> MWSHPQFEKGSMELSYATTMHYRDVVFYVTTDRNRAYFVCGGCVYSVGRPCASQPGEIAKFGLVVRGTGPDDRVVANYVRSELRQRGLQDVRPIGEDEVFLDSVCLLNPNVSSELDVINTNDVEVLDECLAEYCTSLRTSPGVLI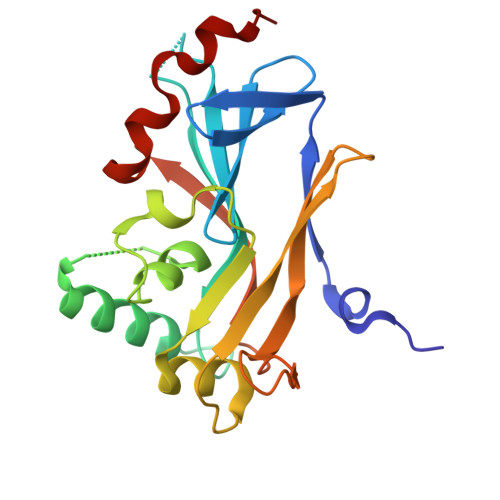SGLRVRAQDRIIELFEHPTIVNVSSHFVYTPSPYVFALAQAHLPRLPSSLEALVSGLFDGIPAP>MASWSHPQFEKGASTSLYKKAGRMSKFTWKELIQLGSPSKAYESSLACIAHIDMNAFFAQVEQMRCGLSKEDPVVCVQWNSIIAVSYAARKYGISRMDTIQEALKKCSNLIPI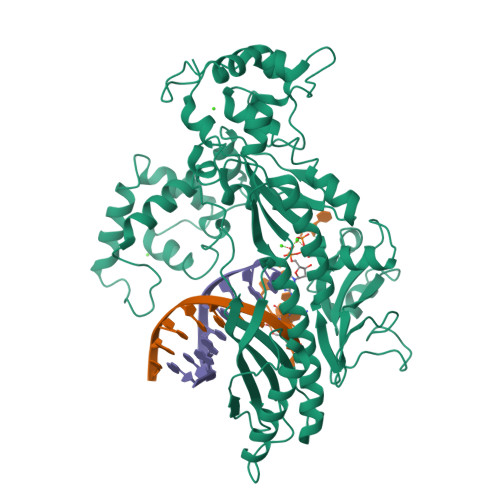HTAVFKKGEDFWQYHDGCGSWVQDPAKQISVEDHKVSLEPYRRESRKALKIFKSACDLVERASIDEVFLDLGRICFNMLMFDNEYELTGDLKLKDALSNIREAFIGGNYDINSHLPLIPEKIKSLKFEGDVFNPEGRDLITDWDDVILALGSQVCKGIRDSIKDILGYTTSCGLSSTKNVCKLASNYKKPDAQTIVKNDCLLDFLDCGKFEITSFWTLGGVLGKELIDVLDLPHENSIKHIRETWPDNAGQLKEFLDAKVKQSDYDRSTSNIDPLKTADLAEKLFKLSRGRYGLPLSSRPVVKSMMSNKNLRGKSCNSIVDCISWLEVFCAELTSRIQDLEQEYNKIVIPRTVSISLKTKSYEVYRKSGPVAYKGINFQSHELLKVGIKFVTDLDIKGKNKSYYPLTKLSMTITNFDIIDLQK[2x]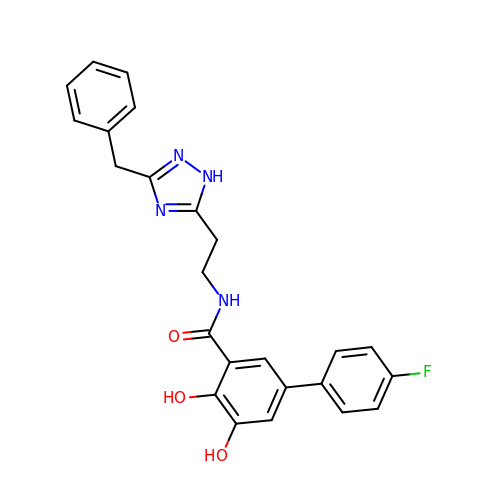N-[2-(5-benzyl-1H-1,2,4-triazol-3-yl)ethyl]-5-(4-fluorophenyl)-2,3-dihydroxybenzamide | C24 H21 F N4 O3 | XLPJSCUSQUKSJT-UHFFFAOYSA-N2-[(5,6-DIPHENYLFURO[2,3-D]PYRIMIDIN-4-YL)AMINO]ETHANOL 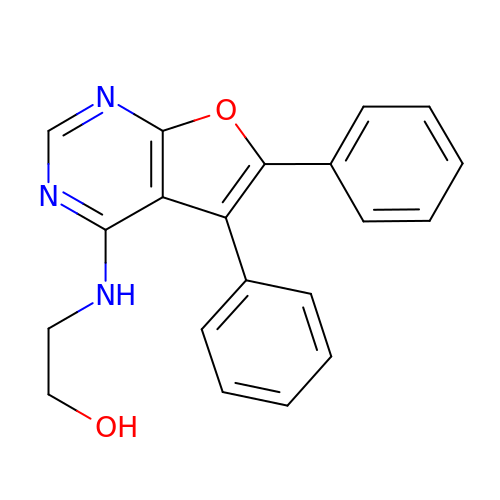| C20 H17 N3 O2 | UQHINZSKNAAVOZ-UHFFFAOYSA-N> TRDQNGTWEMESNENFEGYMKALDIDFATRKIAVRLTQTKVIDQDGDNFKDKTTSTFRNYDVDFTVGVEFDEYTKSLDNRHVKALVTWEGDVLVCVQKGEKENRGWKKWIEGDKLYLELTCGDQVCRQ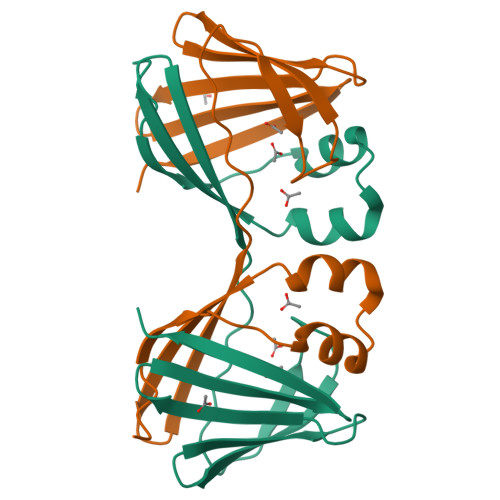VFKKK Here, we focus on the identification and characterization of proteins selectively secreted by the first larval stages of T. suis. We screened a set of n = 6 recombinant larval proteins for immunomodulatory properties and identified an enzymatically active T. suis chitinase that interfered with recruitment of immune cells and inflammatory reactions in a murine model of allergic airway disease. While our in vitro data suggest no direct immunomodulatory effects on, e.g., DC function or T cell activation, we observed disease amelioration to be associated with suppression of eosinophil recruitment into the lung and increased numbers of alternatively activated RELMα+ lung macrophages. Since mammalian host chitinases, both true chitinases with enzymatic activity (AMCase and chitotriosidase) and chitinase-like protein (CLP) molecules which can bind to chitin but lack enzymatic activity, are implicated as either mediators or biomarkers involved in airway inflammation and fibrosis, disease amelioration by treating with a worm chitinase was rather surprising.

The three-dimensional structure of the T. suis chitinase as determined by high-resolution X-ray crystallography revealed high similarities to mouse acidic mammalian chitinase (AMCase) but a unique ability of T. suis chitinase to form dimers. Our data indicate that the structural similarities between the parasite and host chitinase contribute to the disease-ameliorating effect of the helminth-derived chitinase on allergic lung inflammation. Our findings further reveal that T. suis chitinase treatment of allergic mice not only inhibited host AMCase expression on mRNA level but also interfered with host chitinase activity in the BAL fluid, suggesting an alternative mechanism that might involve the high degree of structural similarity between host and nematode chitinases.

>[2x]AAESGARSVCNTVRRRSAGMLRKDSQDASDEKYVRGCYFTNWAQYRPGNGKYNPEHYQANLCEYIFYAFAKLNDDFTVDQFEWNDIDVLYPGVMKQKSSQPDLKVLLSLGGWNAGTATFKKMAATYSNRAKFISSLVSFLQQNKFDGFDLDWEYPESSDKENYLLLCQEILAKFEEVAKCTSTSRLLFTAAVSANPKTVDAGYDVPALAKVLDFVNLMCYDFHGAWETQTGINSPLYSRKEDSSEFKMWNVEQSSKYWSDKGMPKKQIIIGLPTYGRGWTLSDASKTDIGAPAQGSSTATEYLREAGVISYYEVCQKLSSGAKRVWDDESKTPYLVQGNQWFSYDDVESMKAKINWIKQENYGGAFVWTLDYDDFLGSFCTEHNGKKYPLISLMQEILGGGYVPPSTESTTSQVTTTPSTTTSTTSPAGAFQCPSDGLFPDPESCSNFYQCAGGTAYKMKCPTGLMFNPKTSTCDYPSNVDCQEKTITTHHHHHH> SMRAKKMGTVRPWATGLSGQLQKAFVTGVPSLKRSELETACEDFSNIIGSTSTCMLYKGTLSSGVEIAVASSLVTSAKDWSKENESQYRKKITNLSKVSHKNFMNLLGYCEEEHPFTRVMVFEYAPNGTLFEHLHVREAEKLDWMARLRISMGIAYCLEHMHQLQTPAALRNFDSTTVYLTDDFAAKVSDLEFWNDAKGHNSTTNNELAFSPDMEDIVRKYGMVLLEILTGRVPSSEDDGPLENWVSRYFEGGMRLEELIDPSIGFFPEDTARALCEVVRSCIDRDPKKRPQMKEVA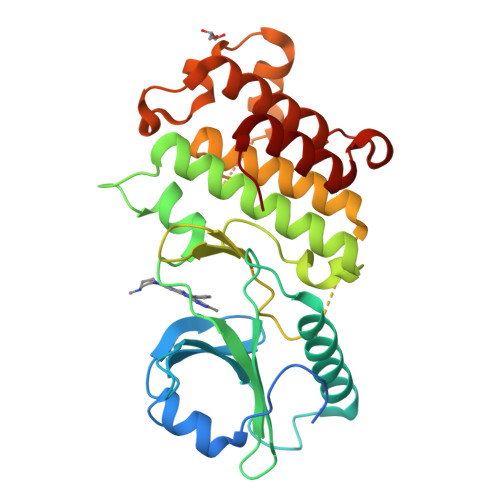ARMREITALGP Group IV sigma factors are known as extracytoplasmic function (ECF) sigma factors, because they are activated in response to extracytoplasmic stresses. The ECF sigma factors are composed of only σ2 and σ4 domains, which bind -10 and -35 elements, respectively. Of these sigma factors, SigW induces the transcription of its target regulon to counteract cell envelope stresses caused by antibiotics, alkaline pH, and high salt concentration. In the absence of these stresses, SigW is downregulated by anti-sigma factor RsiW, which is localized in the plasma membrane.

In the work reported here, we determined the crystal structure of the σW4/-35 element complex, and analyzed the promoter binding mode of SigW. The crystal structure contains a σW4 monomer and a double-stranded -35W in the asymmetric unit. However, residues 125–133, which correspond to α6, are disordered in the crystal structure of σW4/-35W. The residues on α6 are likely to be flexible because they are not bound to DNA directly. α8–α9 of σW4 forms the HTH motif, and α9 is inserted into the major groove of -35W as a DNA recognition helix. The recognition helix α9 mediates the major interactions between σW4 and -35W through hydrogen bonds and hydrophobic interactions. The bases and backbones of three purine nucleotides (G-35 and A-34 in the non-template strand and G’-31’ in the template strand; ‘ indicates the template strand of DNA) form hydrogen bonds with the residues on the N-terminal half of α9 in σW4. Altogether, α9 in σW4 specifically recognizes -35W, and α7-α8 provides additional contacts, leading to a tighter interaction. Like -35E, the narrowing of the minor groove of -35W begins at A-33A-32 and is stabilized downstream of the -35 element, even though the downstream sequence of -35W has an insertion of two cytosines (A-33A-32C-31C-30T-29). The crystal structure of σW4/-35W shows that SigW selectively recognizes cognate -35 promoter elements which have a narrowed minor groove, in a similar manner to the E. coli SigE. Comparison with the SigW/RsiW structure shows that SigW binding to the -35 promoter element and anti-sigma RsiW is mutually exclusive.

> GSLSNTIQQKILKLPDKYRTVIVLKYIDELSLIEIGEILNIPVGTVKTRIHRGREALRKQLRDL>[2x]MDYKDDDDKHMTTSAVNIYNISAGASVDLAAPVTTGDIVTFFSSALNLSAGAGSPN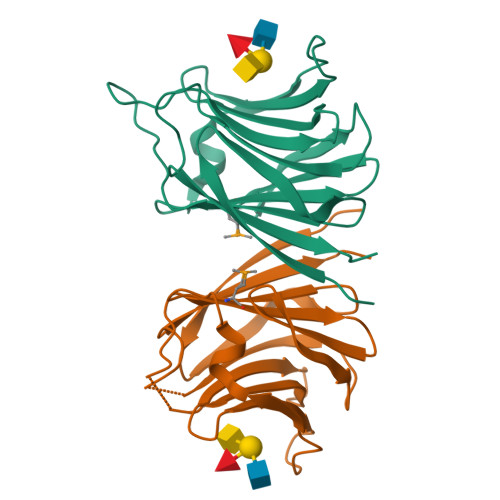NTALNLLSENGAYLLHIAFRLQENVIVFNSRQPNAPWLVEQRVSNVANQFIGSGGKAMVTVFDHGDKYQVVINEKTVIQYTKQISGTTSSLSYNSTEGTSIFSTVVEAVTYTGLAKLAAALE Ubiquitin specific protease 7 (USP7) catalyzes the deubiquitination of many cellular proteins involved in tumor suppression, neural stem cell maintenance, DNA damage and immune responses. USP7 consists of an N-terminal TRAF-like domain (NTD), a catalytic domain (CAT) and five C-terminal ubiquitin-like domains (CTD). In fact USP7 was first discovered through its strong and specific interaction with the ICP0 protein of HSV-1, leading to its original name of Herpesvirus Associated USP (HAUSP). The fact that several proteins bind to the C-terminal ubiquitin-like domains of USP7 prompted us to identify and characterize the interaction mechanism. This study shows the structural basis of interaction between the first three C-terminal ubiquitin-like domains complexed with an ICP0 peptide, revealing a protein binding pocket at Ubl2 of USP7-CTD.

Crystals were only obtained with Ubl123 and ICP0 peptide 617GPRKCARKTRH627. The crystal structure of Ubl123-ICP0 peptide complex was determined to 2.9 Å resolution. The ICP0 peptide binds to a predominantly negatively charged area between 758DELMDGD764 on Ubl2. The two ICP0 lysine residues (K620 and K624) function like a pair of tongs by forming salt-bridges with two buried aspartate residues of USP7 (D762 and D764). These two lysine residues belong to the central part of the peptide (KCARKT), which is in close contact with USP7 due to a backbone-to-backbone hydrogen bond (ICP0 nitrogen-C621 with USP7 oxygen-L760). Interestingly, native Ubl123 crystallized in a previously unknown compact conformation with a direct contact between Ubl1 and Ubl3. A superposition of all available USP7 fragments containing Ubl123 shows two distinct orientations of Ubl3 compared to Ubl12 with a 35 degree motion and a pivot at residue H792. The only strong hydrogen bond between Ubl2 and Ubl3 is formed between the protein backbone of residues H792 and N814. In the compact conformation S814 has moved to the former position of N815, thereby tilting the entire Ubl3 domain against Ubl12. The compact conformation appears to be stabilized by a salt bridge between R871 of Ubl3 and D587 of Ubl1. In the compact conformation of Ubl123, the distance between the catalytic domain and Ubl45 is drastically reduced from 75 Å (extended conformation) to 50 Å.

>MGSSHHHHHHSSGRENLYFQGDIPQQLVERLQEEKRIEAQKRKERQEAHLYMQVQIVAEDQFCGHQGNDMYDEEKVKYTVFKVLKNSSLAEFVQSLSQTMGFPQDQIRLWPMQARSNGTKRPAMLDNEADGNKTMIELSDNENPWTIFLETVDPELAASGATLPKFDKDHDVMLFLKMYDPKTRSLNYCGHIYTPISCKIRDLLPVMCDRAGFIQDTSLILYEEVKPNLTERIQDYDVSLDKALDELMDGDIIVFQKDDPENDNSELPTAKEYFRDLYHRVDVIFCDKTIPNDPGFVVTLSNRMNYFQVAKTVAQRLNTDPMLLQFFKSQGYRDGPGNPLRHNYEGTLRDLLQFFKPRQPKKLYYQQLKMKITDF[2x];>[2x]GPRKCARKTRH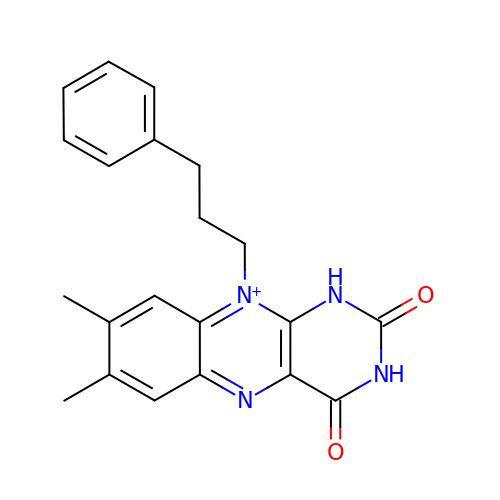7,8-dimethyl-2,4-dioxo-10-(3-phenylpropyl)-1,2,3,4-tetrahydrobenzo[g]pteridin-10-ium | C21 H21 N4 O2 | LVUMBLZQGDFTPC-UHFFFAOYSA-O>PLTDTDRSEDFLRRVRGLKAARTANGPRLYQPITLLWAVGRARRGEARTLAWADTDEAIGALLKRHGARGERPRPDYPVLALHRAGLWTLEGHVGEVPTAHGDSALRNWFAEQRPVGGLAEPFHDLLHR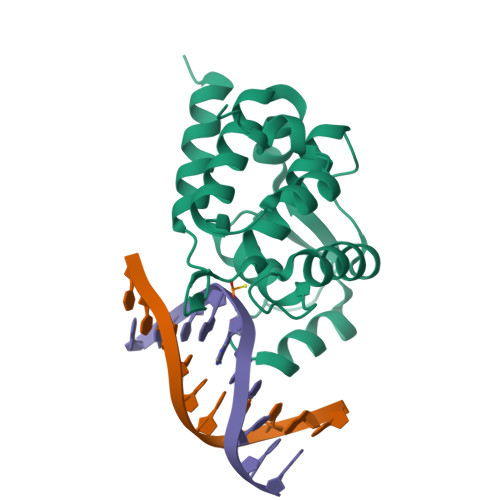SGHSRVSVIEALLTTYFAGLDPVPLLEDTGLYDEGHHHHH[2x]> ADTGPALKAGHEYMIVTNYPNNLHVVDVASDTVYKSCVMPDKFGPGTAMMAPDNRTAYVLNNHYGDIYGIDLDTCKNTFHAN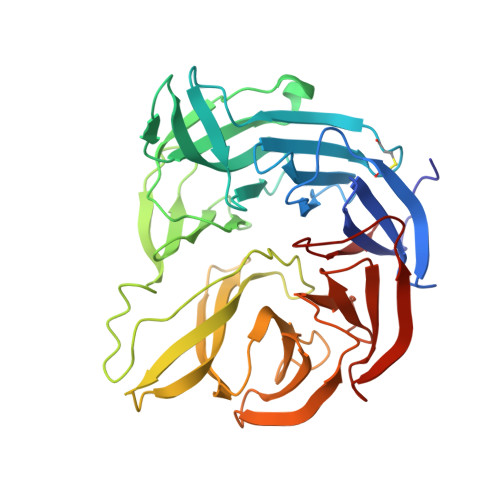LSSVPGEVGRSMYSFAISPDGKEVYATVNPTQRLNDHYVVKPPRLEVFSTADGLEAKPVRTFPMPRQVYLMRAADDGSLYVAGPDIYKMDVKTGKYTVALPLRNWNRKGYSAPDVLYFWPHQSPRHEFSMLYTIARFKDDKQDPATADLLYGYLSVDLKTGKTHTQEFADLTELYFTGLRSPKDPNQIYGVLNRLAKYDLKQRKLIKAANLDHTYYCVAFDKKGDKLYLGGTFNDLAVFNPDTLEKVKNIKLPGGDMSTTTPQVFIR>GVACKPKEKPSSATSLTDDALMDTVQRRTFNYFWDAAEPNSGLARERYHMDGEYPAGGPEIVTSGGSGFGIMAILAGIDRGYVSREEGLRRMEKIVGFLEKADRFKGAYPHWWNGETGHVQPFGQKDNGGDLVETAFLMQGLLAVHQYYAEGSAEEKKLAGRIDKLWREVDWNWYRHGGQNVLYW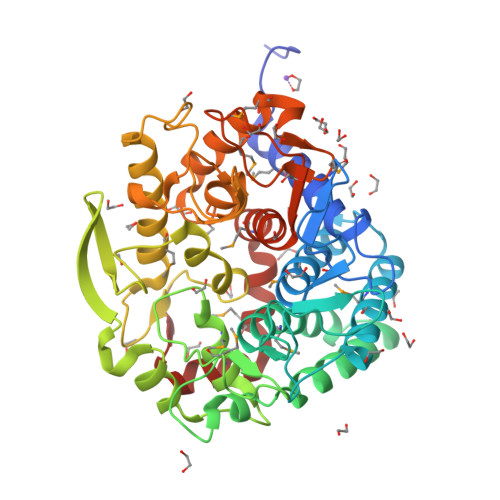HWSPEYGWEMNFPVHGYNECLIMYILAAASPTHGVPAAVYHEGWAQNGAIVSPHKVEGIELHLRYQGGEAGPLFWAQYSFLGLDPVGLKDEYCPSYFNEMRNLTLVNREYCIRNPKHYKGYGPDCWGLTASYSVDGYAAHGPLERDDRGVISPTAALSSIVYTPDQSLQVMHHLYEMGDKVFGPYGFYDAFSETADWYPKRYLAIDQGPIAVMIENYRTGLLWKLFMSHPDVQNGLKKLGFNVKK[4x]> IWELKKDVYVVELDWYPDAPGEMVVLTCDTPEEDGITWTLDQSSEVLGSGKTLTIQVKE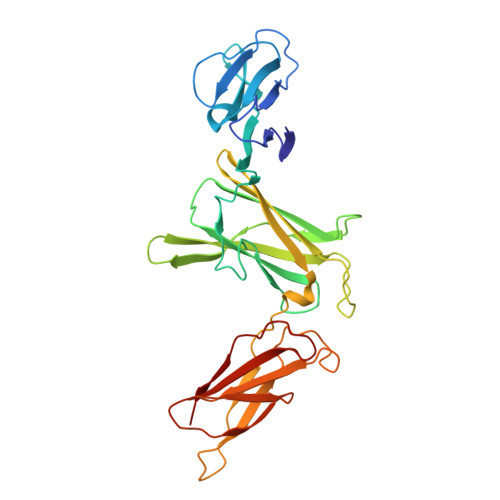FGDAGQYTCHKGGEVLSHSLLLLHKKEDGIWSTDILKDQKEPKNKTFLRCEAKNYSGRFTCWWLTTISTDLTFSVKSSRGSSDPQGVTCGAATLSAERVRGDNKEYEYSVECQEDSACPAAEESLPIEVMVDAVHKLKYEQYTSSFFIRDIIKPDPPKNLQLKPLKNSRQVEVSWEYPDTWSTPHSYFSLTFCVQVQGKSKREKKDRVFTDKTSATVICRKNASISVRAQDRYYSSSWSEWASVPCS>[2x]SNAEKEKDTIAAEHKQEASVLLNLHRNKINYLIGETMARMTSLSIAIDRPVDIKKMQSILEKTFDSEPRFSGLYFLNAKGDVTASTTELKTKVNLADRSFFIKAKETKKTVIS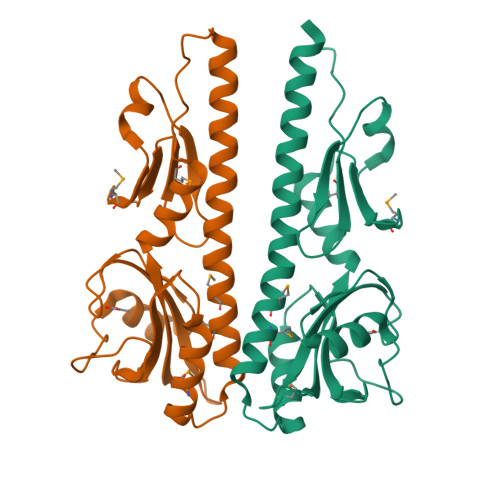DSYSSRITGQPIFTICVPVLDSKRNVTDYLVAAIQIDYLKNLINLLSPDVYIEVVNQDGKMIFASGQASHAEDQKPVSGYLDDISWNMKVYPNPVTIEELSKSL>[2x]MDYKDDDDKHHHHHHENLYFQGMPTNFTVVPVEAHADGGGDETAERTEAPGTPEGPEPERPSPGDGNPRENSPFLNNVEVEQESFFEGKNMALFEEEMDSNPMVSSLLNKLANYTNLSQGVVEHEEDEESRRREAKAPRMGTFIGVYLPCLQNILGVILFLRLTWIVGVAGVLESFLIVAMCCTCTMLTAISMSAIATNGVVPAGGSYYMISRSLGPEFGGAVGLCFYLGTTFAGAMYILGTIEIFLTYISPGAAIFQAEAAGGEAAAMLHNMRVYGTCTLVLMALVVFVGVKYVNKLALVFLACVVLSILAIYAGVIKSAFDPPDIPVCLLGNRTLSRRSFDACVKAYGIHNNSATSALWGLFCNGSQPSAACDEYFIQNNVTEIQGIPGAASGVFLENLWSTYAHAGAFVEKKGVPSVPVAEESRASALPYVLTDIAASFTL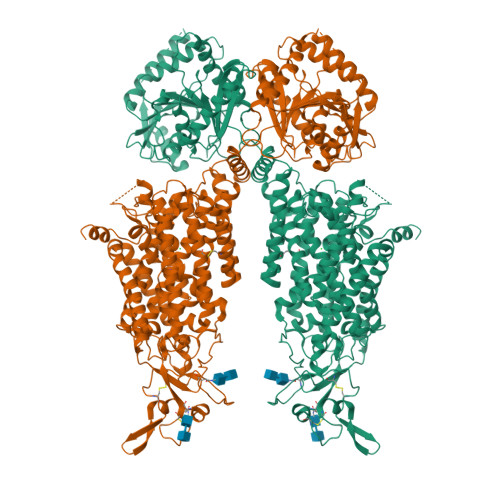LVGIYFPSVTGIMAGSNRSGDLKDAQKSIPTGTILAIVTTSFIYLSCIVLFGACIEGVVLRDKFGEALQGNLVIGMLAWPSPWVIVIGSFFSTCGAGLQSLTGAPRLLQAIARDGIVPFLQVFGHGKANGEPTWALLLTVLICETGILIASLDSVAPILSMFFLMCYLFVNLACAVQTLLRTPNWRPRFKFYHWTLSFLGMSLCLALMFICSWYYALSAMLIAGCIYKYIEYRGAEKEWGDGIRGLSLNAARYALLRVEHGPPHTKNWRPQVLVMLNLDAEQAVKHPRLLSFTSQLKAGKGLTIVGSVLEGTYLDKHMEAQRAEENIRSLMSTEKTKGFCQLVVSSSLRDGMSHLIQSAGLGGLKHNTVLMAWPASWKQEDNPFSWKNFVDTVRDTTAAHQALLVAKNVDSFPQNQERFGGGHIDVWWIVHDGGMLMLLPFLLRQHKVWRKCRMRIFTVAQVDDNSIQMKKDLQMFLYHLRISAEVEVVEMVENDISAFTYERTLMMEQRSQMLKQMQLSKNEQEREAQLIHDRNTASHTAAAARTQAPPTPDKVQMTWTREKLIAEKYRSRDTSLSGFKDLFSMKPDQSNVRRMHTAVKLNGVVLNKSQDAQLVLLNMPGPPKNRQGDENYMEFLEVLTEGLNRVLLVRGGGREVITIYSWSHPQFEK>[2x]G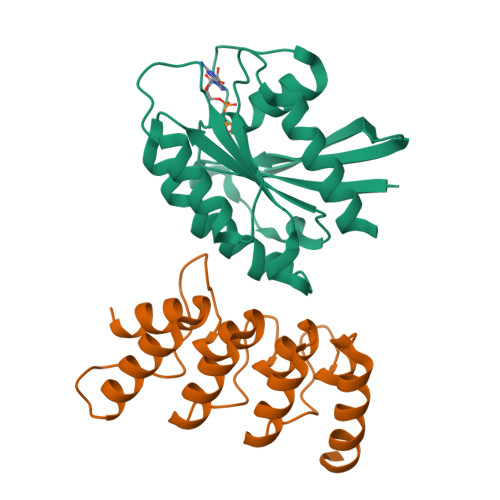SAMGSTSRKKVLLKVIILGDSGVGKTSLMNQYVNKKFSNQYKATIGADFLTKEVMVDDRLVTMQIWDTAGLERFQSGVAFYRGADCCVLVFDVTAPNTFKTLDSWRDEFLIQASPRDPENFPFVVLGNKIDLENRQVATKRAQAWCYSKNNIPYFETSAKEAINVEQAFQTIARNALKQETEVELYNEFPEPIKLDKN;>[2x]GSAMGSAEQQLLHHARNGNAEEVRQLLETMARNEVIADINCKGRSKSNLGWTPLHLACYFGHRQVVQDLLKAGAEVNVLNDMGDTPLHRAAFTGRKELVMLLLEYNADTTIVNGSGQTAKEVTHAEEIRSMLEAVERTQQRKLEELLLAAAREG(4~{a}~{S},8~{a}~{R})-2-cycloheptyl-4-[4-methoxy-3-[2-(2-oxidanylideneimidazolidin-1-yl)ethoxy]phenyl]-4~{a},5,8,8~{a}-tetrahydrophthalazin-1-one 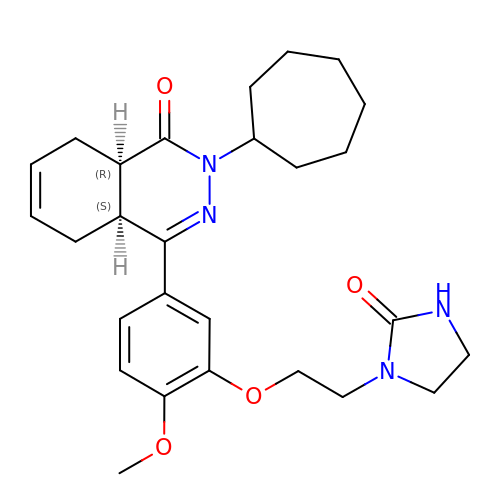| C27 H36 N4 O4 | YLCZKQRIIGKMHV-FCHUYYIVSA-N>[2x]MTRHHHHHHGGGDYKDDDDKGGGKVPVEEEIQDLKAVWVELSNTWQEIDSLKETAWSAIIPRKVRKSLEDTLQKLKNLPNRIRQYSAFDHAQNLIKIYLKGNAIITDLHSEAIKDRHWKILKKRLNTNWIITELTLGSIWDSDLARNENIYREVITAAQGEIALEEFLKGVREFWTTLELDLVNYQRKCKLVRGWDDLFNKLAEHLNSISAMKMSPYYKVFEEEANHWDDRLNKVRSLLDVWIDVQRRWVYLEGIFSGSGDINQLLPAESTRFKSINSEFIAILKKVSGAPLILEVLAIERIQQTMERLSDLLGKVQKALGEYLERQRSAFARFYFVGDEDLLEIIGNSKDIIKIQKHFRKMFAGLANLTLDDEKTTIIGMSSAEGETVTFKKPISIANGPKIHEWLTMVESEMKSTLATLLSESLQHFNQVDVNDHSKYSEWVDNYPTQLVLLTSQIVWSTQVDQALGGGTLQQSKIQEQLQSIEQTTQMILNNLADSVLQDLSAQKRKKFEHLITELVHQRDVVRQLQKCKNLTGNKDFDWLYHMRYYYDATQENVLHKLVIHMANATFYYGFEYLGIGERLVQTPLTDRCYLTLTQALESRMGGNPFGPAGTGKTETVKALGSQLGRFVLVFCCDEGFDLQAMSRIFVGLCQCGAWGCFDEFNRLEERILSAVSQQIQTIQVALKENSKEVELLGGKNISLHQDMGIFVTMNPGYAGRSNLPDNLKKLFRSMAMIKPDREMIAQVMLYSQGFKTAEVLAGKIVPLFKLCQEQLSAQSHYDFGLRALKSVLVSAGGIKRKCQPPQLPPITDAESKTKADQIYCQYEIGVLLNSINDTMIPKLVADDIPLIQSLLLDVFPGSQLQPIQMDQLRKKIQEIAKQRHLVTKQEWVEKILQLHQILNINHGVMMVGPSGGGKT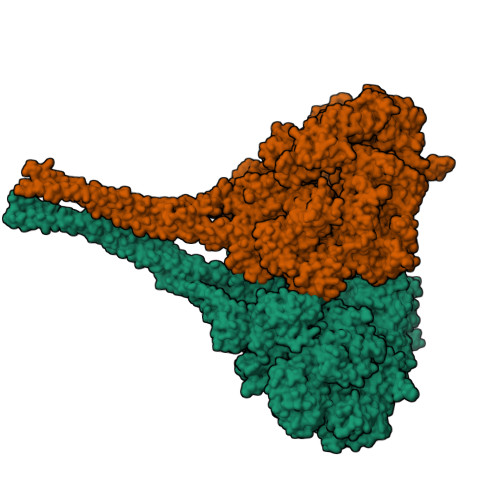TSWEVYLEAIEQVDNIKSEAHVMDPKAITKDQLFGSLDLTTREWTDGLFTATLRRIIDNVRGESTKRHWIIFDGDVDPEWVENLNSLLDDNKLLTLPNGERLALPNNVRVMFEVQDLKYATLATISRCGMVWFSEEILTTQMIFQNYLDTLSNEPFDPQEKEQQKRNENAQLQQQQQTTITSPILTSPPTTSSSSRSTTSTTSMIPAGLKVQKECAAIISQYFEPGGLVHKVLEDAGQRPHIMDFTRLRVLNSFFSLMNRSIVNVIEYNQLHSDFPMSPENQSNYITNRLLYSLMWGLGGSMGLVERENFSKFIQTIAITPVPANTIPLLDYSVSIDDANWSLWKNKVPSVEVETHKVASPDVVIPTVDTTRHVDVLHAWLSEHRPLILCGPPGSGKTMTLTSTLRAFPDFEVVSLNFSSATTPELLLKTFDHHCEYKRTPSGETVLRPTQLGKWLVVFCDEINLPSTDKYGTQRVITFIRQMVEKGGFWRTSDHTWIKLDKIQFVGACNPPTDAGRVQLTHRFLRHAPILLVDFPSTSSLTQIYGTFNRALMKLLPNLRSFADNLTDAMVEFYSESQKRFTPDIQAHYIYSPRELSRWDRALLEAIQTMDGCTLEGLVRLWAHEALRLFQDRLVETEEKEWTDKKIDEVALKHFPSVNLDALKRPILYSNWLTKDYQPVNRSDLREYVKARLKVFYEEELDVPLVLFNEVLDHILRIDRVFRQPQGHALLIGVSGGGKSVLSRFVAWMNGLSIYTIKVNNNYKSSDFDDDLRMLLKRAGCKEEKICFIFDESNVLESSFLERMNTLLAGGEVPGLFEGEEFTALMHACKETAQRNGLILDSEEELYKYFTSQVRRNLHVVFTMNPASPDFHNRSATSPALFNRCVLDWFGEWSPEALFQVGSEFTRNLDLENPQYIAPPVFIQEAEIMGNNLMAIPPSHRDAVVSSLVYIHQTIGEANIRLLKRQGRQNYVTPRHYLDFINQVVLLINEKRDQLEEEQLHLNIGLKKLRDTEAQVKDLQVSLAQKNRELDVKNEQANQKLKQMVQDQQAAEIKQKDARELQVQLDVRNKEIAVQKVKAYADLEKAEPTGPLREEVEQLENAANELKLKQDEIVATITALEKSIATYKEEYATLIRETEQIKTESSKVKNKVDRSIALLDNLNSERGRWEQQSENFNTQMSTVVGDVVLASAFLAYIGFFDQNFRTDLMRKWMIRLDSVGIKFKSDLSVPSFLSKPEERLNWHANSLPSDELCIENAIMLKRFNRYPLVIDPSGQAMEFLMNQYADKKITKTSFLDSSFMKNLESALRFGCPLLVQDVENIDPVLNPVLNKEIRKKGGRILIRLGDQDVDFSPSFMIFLFTRDPTAHFTPDLCSRVTFVNFTVTPSSLQSQCLHEALKTERPDTHKKRSDLLKIQGEFQVKLRILEKSLLNALSQASGNILDDDSVISTLETLKKETTEIALKVEETETVMQEISEVSALYNPMALSCSRVYFAMEELSQFHLYQFSLRAFLDIFYNLLNNNPNLVDKKDPNERLVYLSKDIFSMTFNRVTRTLLNDDKLTFALQLTIISVKGTSNEIEESEWDFLLKGGDNLTSIKETIPQLDSLLSTTQQKWLICLRQQVPSFSKLVDHIQQNSSDWKQFFGKDQVGEPIIPESWIVAQAQLSNQQSTIVSNFRKILLMKAFHSDRVLQYSHSFVCSVFGEDFLNTQELDMANIVEKEVKSSSPLLLCSVPGYDASSKVDDLALQLHKQYKSFAIGSPEGFELAEKSIYAAAKSGTWVLLKNIHLAPQWLVQLEKKLHSLSPHPSFRLFMTSEIHPALPANLLRMSNVFSYENPPGVKANLLHTFIGIPATRMDKQPAERSRIYFLLAWFHAIIQERLRYIPLGWTKFFEFNDADLRGALDSIDYWVDLYSKGRSNIDPDKIPWIAVRTILGSTIYGGRIDNEFDMRLLYSFLEQLFTPSAFNPDFPLVPSIGLSVPEGTTRAHFMKWIEALPEISTPIWLGLPENAESLLLSNKARKMINDLQKMQSSEEDGEDDQVSGSSKKESSSSSSEDKGKAKLRATITEWTKLLPKPLKQLKRTTQNIKDPLFRCFEREISTGGKLVKKITNDLANLLELISGNIKSTNYLRSLTTSISKGIVPKEWKWYSVPETISLSVWISDFSKRMQQLSEISESSDYSSIQVWLGGLLNPEAYITATRQSASQLNGWSLENLRLHASSLGKISSEGGASFNVKGMALEGAVWNNDQLTPTDILSTPISIATLTWKDKDDPIFNNSSSKLSVPVYLNETRSELLFSIDLPYDQSTSKQNWYQRSVSISSWKSDI> G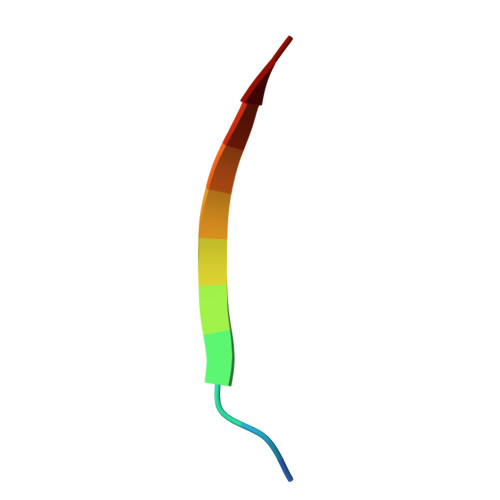VKSLKRRRCY3-[(3-{[3-(METHYLAMINO)PROPYL]AMINO}PROPYL)AMINO]PROPANE-1,1-DIOL 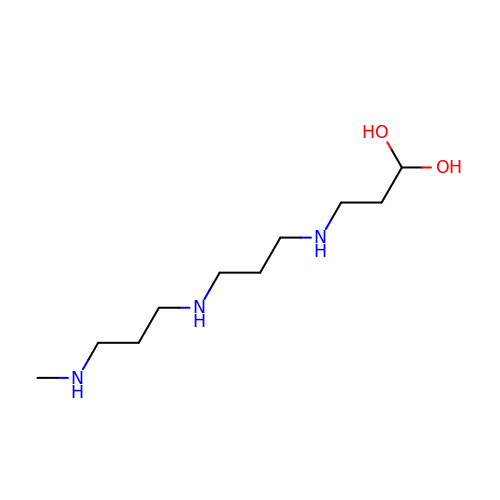| C10 H25 N3 O2 | PTLIEDFKZYQZEI-UHFFFAOYSA-N Uridine 5'Diphospho N-acetyl 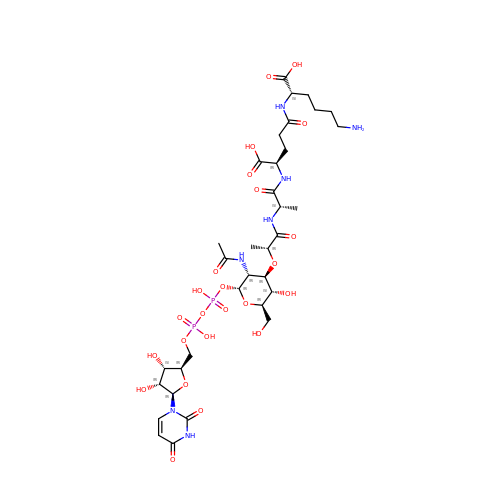muramoyl-L-Alanyl-D-Glutamyl-L-Lysine | C34 H55 N7 O24 P2 | WXBLSQNZKMJACT-BYEZXYKXSA-N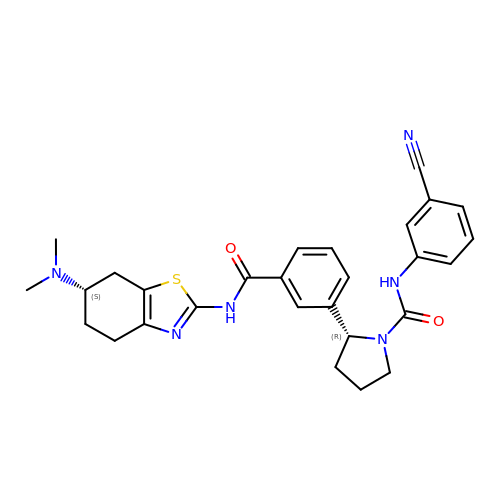(2R)-N-(3-cyanophenyl)-2-(3-{[(6S)-6-(dimethylamino)-4,5,6,7-tetrahydro-1,3-benzothiazol-2-yl]carbamoyl}phenyl)pyrrolidine-1-carboxamide | C28 H30 N6 O2 S | HOQOXPZIFORKKX-LADGPHEKSA-N> MAAAAPNAGGSAPETAGSAEAPLQYSLLLQYLVGDKRQP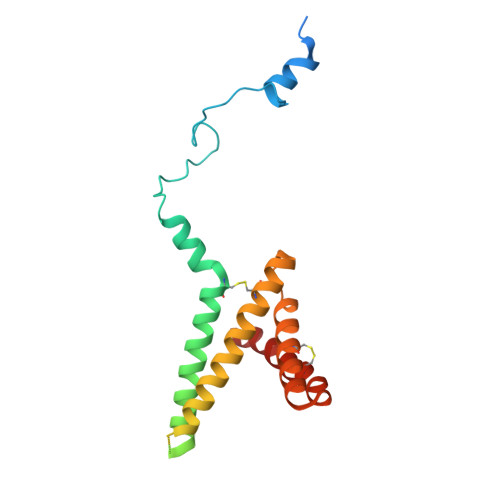RLLEPGSLGGIPSPAKSEEQKMIEKAMESCAFKAALACVGGFVLGGAFGVFTAGIDTNVGFDPKDPYRTPTAKEVLKDMGQRGMSYAKNFAIVGAMFSCTECLIESYRGTSDWKNSVISGCITGGAIGFRAGLKAGAIGCGGFAAFSAAIDYYLR> TSSATSSSSMILKYPYRVVDTHEKLKEAVTSLQGARSIALDIEAFCTTDQAKQLGRISLVQACSDAKPVVFLFDVLTLTPDVFVKDMQSLLSDREIRKLFFDCRRDVEALSCQLGVKPEGVLDLQVFFTAIQWKLRSVNRRSGMGYVLKSVAGLTRQEGDSAVQTAMTLGNRPVWDIRPLPDHFLEYAAGDVRHILLLSNYLVGNKDVPVDVVAVERLTAQYVEHYAVGKPVITEADATPAEVNRAWLERYIGPGGGCHFCGAKGHTEAECFKKQNGKAKCSFCGEVGHTARNCFKKHPQLLTCEKCGQLGHTGTSCFRTNPCKHCGGPHSSANCHKVIWQQKRLGENSLH

Compared to TbREX1, TbREX2 and TbDSS-1, TbRND is unique, as it belongs to the RNase D (RND) group within the DEDD exoribonuclease superfamily. Like E. coli RNase D (EcRND), Saccharomyces cerevisiae Rrp6 (ScRrp6), and all other RND family proteins, TbRND possesses a single 3′-5′ exoribonuclease (Exo) domain. EcRND and ScRrp6 possess an HRDC (helicase and RNase D C-terminal) domain at the C-termini whereas TbRND contains a predicted CCHC zinc-finger domain (ZFD) at its C-terminus. Depletion of TbRND results in extended gRNA tails in vivo, whereas, overexpression of TbRND leads to a substantial reduction in the total gRNA population and the subsequent inhibition of mRNA editing.

Like the G-form structure, the ZFD also adopts an extended conformation in the Apo-form structure. Structural analysis suggested that the extended ZFD conformations are mainly stabilized by crystal packing. Although ZF3 and ZF4 are also present in the Apo-form structure, they are disordered, suggesting that they don’t form stable interactions with surrounding molecules. In contrast, ZF2 is well defined in both structures, due to its extensive interactions with symmetry-related molecules. In the presence of RNA-12U, Arg179 and Phe311 pack against the RNA and adopt a stable conformation, while in the absence of RNA, the side chains of Arg179 and Phe311 are disordered and flexible, as indicated by their high B-factors and weak electron densities. Interestingly, however, the relative orientations between the Exo domain and ZF1 are very similar in the Apo-form and RNA-complexed structures of TbRND. ZF2 adopts an extended conformation in the Apo-form and the G-form structures.> GAMARVGPKIEITHGGKKYTVFSKV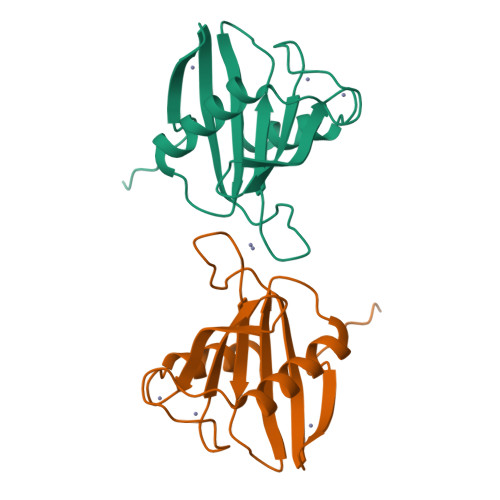THLVPRTENGEEAEYVVFGPEKEGVISVVVLAPKDLNEEALALRVKWFNDTKPRCVKCGAAYNGKNHFRVVAIRNGTYYLDAVCDKCEPRITWLSAIVIGRS> MNRNVYAVLSTVLAASLLAACNSGGEQVKAESKNKTAATQQSEPNVIAAHKGVNQAPVPLKMERVGPHDVHIEMTAQITDIEIDKGKIYKAWTFNGQAPGPLVVVNEGDTIHFTLKNMDPVVPHSMD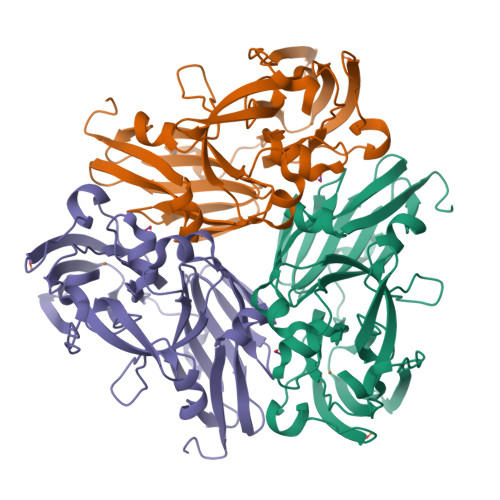FHAVHASPSKDFIDVMPNKSGTFTYPANKPGVFMYHAGTKPVLQHIANGMHGVIIVKPKNGYPTDKEVDREYVLIQNEWYKYNDMNDFQNGVPSYVVFSSKALKPGDPNTNGDTFTLKEKPLLAKVGEKIRLYINNVGPNEVSSFHVVGTVFDDVYLDGNPNNHLQGMQTVMLPASGGAVVEFTVTRPGTYPIVTHQFNHAQKGAVAMLKVTETGEDDGTETSGH> MSSLQKRPGPGNSSQPTERPRKESILDLSRYQDQRIQATFT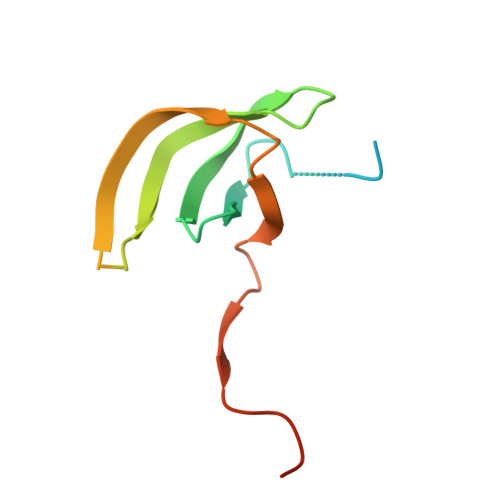GGRQITGILKGFDQLMNLVLDDVEEQLRNPEDGKLTGAIRKLGLVVVRGTTLVLIAPMDGSEEIPNPFVQAEHHHHHH> SLTSADKSHVKSI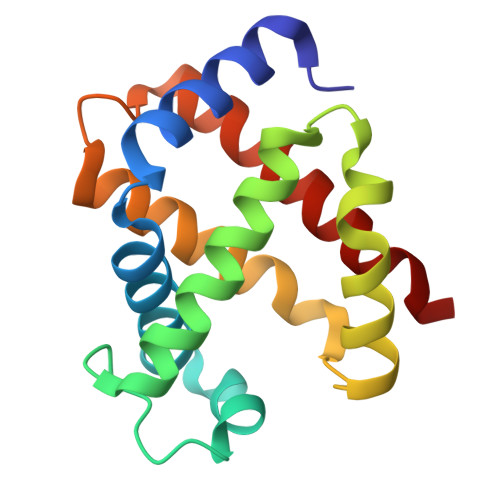WSKASGKAEELGAEALGRMLEVFPNTKTYFSHYADLSVSSGQVHTHGKKILDAITTAVNHIDDITGTMTALSTLHAKTLRVDPANFKILSHTILVVLALYFPADFTPEVHLACDKFLASVSHTLATKYR>[4x]MHHHHHHLEPPPSTFQPLCHPLVEEVSKEVDGYFLQHWNFPNEKARKKFVAAGFSRVTCLYFPKALDDRIHFACRLLTVLFLIDDLLEYMSFEEGSAYNEKLIPISRGDVLPDRSIPVEYIIYDLWESMRAHDREMADEILEPVFLFMRAQTDRTRARPMGLGGYLEYRERDVGKELLAALMRFSMGLKLSPSELQRVRE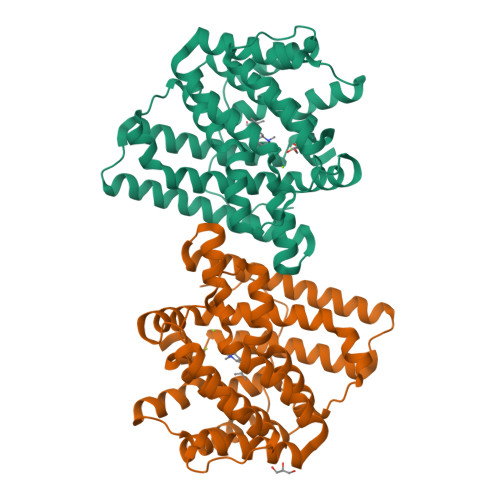IDANCSKHLSVVNDIYSYEKELYTSKTAHSEGGILCTSVQILAQEADVTAEAAKRVLFVMCREWELRHQLLVARLSAEGLETPGLAAYVEGLEYQMSGNELWSQTTLRYSVVVD>MQRKTFADAECPIARSLERVGEWWSILIMRDALQGLRRFDEFSRSLDIAPNMLTRRLNALVEAGLLERQPYSQRPLRYQYVPTAKGEDFRVVLMAFVAWGNRHYAQQGQSVQLVERTSGRPVRSFMAALADGRTVPLEQCTVQAGPAASEEMRQRLAAMPERSELPAR[12x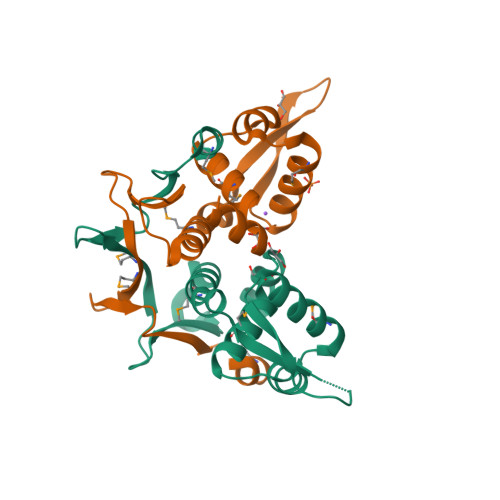]>MPHFTVVPVDGPRRGDYDNLEGLSWVDYGERAELDDSDGHGNHRESSPFLSPLEASRGIDYYDRNLALFEEELDIRPKVSSLLGKLVSYTNLTQGAKEHEEAESGEGTRRRAAEAPSMGTLMGVYLPCLQNIFGVILFLRLTWMVGTAGVLQALLIVLICCCCTLLTAISMSAIATNGVVPAGGSYFMISRSLGPEFGGAVGLCFYLGTTFAAAMYILGAIEILLTYIAPPAAIFYPSGAHDTSNATLNNMRVYGTIFLTFMTLVVFVGVKYVNKFASLFLACVIISILSIYAGGIKSIFDPPVFPVCMLGNRTLSRDQFDICAKTAVVDNETVATQLWSFFCHSPNLTTDSCDPYFMLNNVTEIPGIPGAAAGVLQENLWSAYLEKGDIVEKHGLPSADAPSLKESLPLYVVADIATSFTVLVGIFFPSVTGIMAGSNRSGDLRDAQKSIPVGTILAIITTSLVYFSSVVLFGACIEGVVLRDKYGDGVSRNLVVGTLAWPSPWVIVIGSFFSTCGAGLQSLTGAPRLLQAIAKDNIIPFLRVFGHGKVNGEPTWALLLTALIAELGILIASLDMVAPILSMFFLMCYLFVNLACAVQTLLRTPNWRPRFKYYHWALSFLGMSLCLALMFVSSWY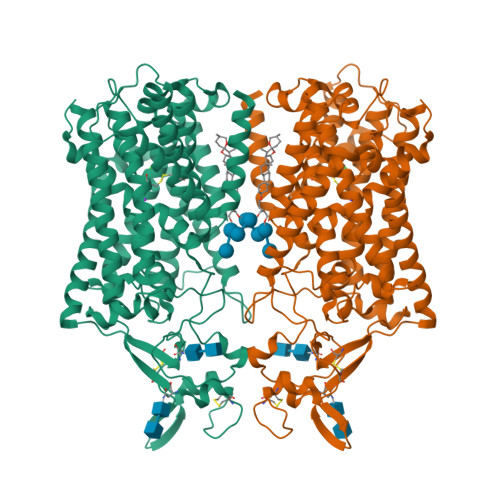YALVAMLIAGMIYKYIEYQGAEKEWGDGIRGLSLSAARYALLRLEEGPPHTKNWRPQLLVLLKLDEDLHVKYPRLLTFASQLKAGKGLTIVGSVIQGSFLESYGEAQAAEQTIKNMMEIEKVKGFCQVVVASKVREGLAHLIQSCGLGGMRHNSVVLGWPYGWRQSEDPRAWKTFIDTVRCTTAAHLALLVPKNIAFYPSNHERYLEGHIDVWWIVHDGGMLMLLPFLLRQHKVWRKCRMRIFTVAQMDDNSIQMKKDLAVFLYHLRLEAEVEVVEMHNSDISAYTYERTLMMEQRSQMLRQMRLTKTEREREAQLVKDRHSALRLESLYSDEEDESAVGADKIQMTWTRDKYMTETWDPSHAPDNFRELVHIKPDQSNVRRMHTAVKLNEVIVTRSHDARLVLLNMPGPPRNSEGDENYMEFLEVLTEGLERVLLVRGGGREVITIYSLEWSHPQFEK[2x]>[2x]MKINDDIKELILEYMSRYFKFENDFYKLPGIKFTDANWQKFKNGGTDIEKMGAARVNAMLDCLFDDFELAMIGKAQTNYYNDNSLKMNMPFYTYYDMFKKQQLLKWLKNNRDDVIGGTGRMYTASGNYIANAYLEVALESSSLGSGSYMLQMRFKDYSKGQEPIPSGRQNRLEWIENNLENIR

Expression of the putative acr on a plasmid in a CR1-immunized S. thermophilus strain completely abolished immunity against the CRISPR-sensitive virulent phage D5842 (green), and even eliminated the residual resistance observed against phage D1811 (red). This new Acr, which bears no similarity to any Acr characterized to date, was named AcrIIA6. All AcrIIA6 and AcrIIA5 orthologs completely restored the plaquing efficiency of phages targeted by the CR1 system of S. thermophilus, indicating they are blocking the activity of St1Cas9. AcrIIA6s did not impede SpCas9, while AcrIIA2 and AcrIIA4 exhibited only a partial inhibition.

Gel filtration profiles also indicated that AcrIIA6 is a dimer in solution. Each monomer consists of eight α-helices and four β-strands forming a β-sheet, with the sequence topology α1α2α3α4α5α6α7β1β2β3β4α8. The superimposition of the AcrIIA6 HTH dimer onto the C.Esp1396I-dsDNA complex brings the AcrIIA6 helix 3 into contact with the two major grooves of the dsDNA. Helix 3 exhibits strong electropositivity, a feature observed in dsDNA binding helices, including the one from C.Esp1396I. We mapped the sequence conservation among the 48 unique AcrIIA6 alleles to the structure obtained. The dimerization interface is largely conserved as are the DNA-interacting arms of the HTH motif.> MNQTDTSPIRLRRSWNTSEIEALFDEHAGRIDPRIYTDEDLYQLELERVFARSWLLLGHETQIRKPGDYITTYMGEDPVVVVRQKDASIAVFLNQCRHRGMRICRADAGNAKAFTCSYHGWAYDTAGNLVNVPYEAESFACLNKKEWSPLKARVETYKGLIFANWDENAVDLDTYLGEAKFYMDHMLDRTEAGTEAIPGVQKWVIPCNWKFAAEQFCSDMYHAGTTSHLSGILAGLPEDLEMADLAPPTVGKQYRASWGGHGSGFYVGDPNLMLAIMGPKVTSYWTEGPASEKAAERLGSVERGSKLMVEHMTVFPTCSFLPGINTVRTWHPRGPNEVEVWAFTVVDADAPDDIKEEFRRQTLRTFSAGGVFEQDDGENWVEIQHILRGHKARSRPFNAEMSMDQTVDNDPVYPGRISNNVYSEEAARGLYAHWLRMMTSPDWDALKATR;> MIDSANRADVFLRKPAPVAPELQHEV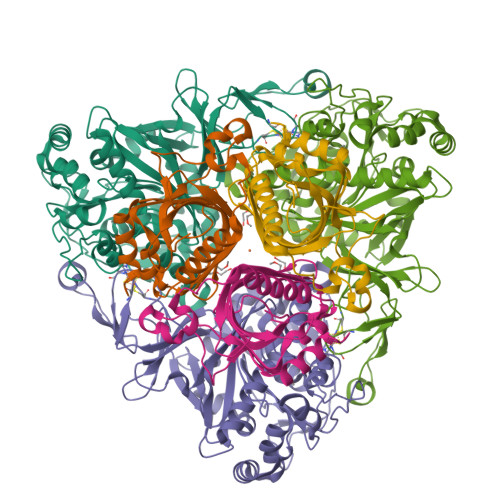EQFYYWEAKLLNDRRFEEWFALLAEDIHYFMPIRTTRIMRDSRLEYSGSREYAHFDDDATMMKGRLRKITSDVSWSENPASRTRHLVSNVMIVGAEAEGEYEISSAFIVYRNRLERQLDIFAGERRDTLRRNTSEAGFEIVNRTILIDQSTILANNLSFFF>SRCTHLENRDFVTGTQGTTRVTLVLELGGCVTITAEGKPSMDVWLDAIYQENPAKTREYCLHAKLSDTKVAARCPTMGPATLAEEHQGGTVCKRDQSDRGWGNHCGLFGKGSIVACVKAACEAKKKATGHVYDANKIVYTVKVEPHTGDYVAANETHSGRKTASFTVSSEKTILTMGEYGDVSLLCRVASGVDLAQTVILELDKTVEHLPTAWQVHRDWFNDLALPWKHEGAQNWNNAERLVEFGAPHAVKMDVYNLGDQTGVLLKALAGVPVAHIEGTKYHLKSGHVTCEVGLEKLKMKGLTYTMCDKTKFTWKRAPTDSGHDTVVMEVTFSGTKPCRIPVRAVAHGSPDVNVAMLITPNPTIENNGGGFIEMQLPPGDNIIYVGELSHQWFQKGSSIGRVFQKTKKGIERLTVIGEHAWDFGSAGGFLSSIGKAVHTVLGGAFNSIFGGVGFLPKLLLGVALAWLGLNMRNPTMSMSFLLAGGLVLAMTLGVGA[3x];>[3x]TVRKERDGSTVIRAEGKDAATQVRVENGTCVILATDMGSWCDDSLSYECVTIDQGEEPVDVDCFCRNVDGVYLEYGRCGKQEGSRTRRSVLIPSHAQGELTGRGHKWLEGDSLRTHLTRVEGWVWKNKLLALAMVTVVWLTLESVVTRVAVLVVLLCLAPVYA

The envelope of immature TBEV particle contains 180 copies of each M protein precursor (prM) and E forming heterodimers. The prM protein stabilizes E, preventing premature virus activation and its fusion at low pH with the membranes of the trans-Golgi network (TGN). Flavivirus maturation occurs at mildly acidic pH, when host protease furin cleaves the prM protein to a pr peptide that will later dissociate from the particle and the M protein that remains in the particle, resulting in infectious viruses. Our atomic models of the major viral components, the E and prM proteins, indicate that the pr domains of prM have a critical role in holding the heterohexameric prM3E3 spikes in a metastable conformation.

(B) Atomic model of a Kuutsalo-14 prM3E3 spike refined against a 3.9-Å-resolution map. We observed a 1.0-Å root-mean-square deviation (RMSD) between Kuutsalo-14 and Neudoerfl atomic models for the Cα of prM and E ectodomains. The E ectodomains extend outward from the particle surface joining at the top like a tripod, with the pr domains of prM positioned at the top. The E-DII harboring the fusion loops join at the top of the prM3E3 spike and are capped by pr peptides, each of which binds to its respective E through an interface with a cumulative buried area of ~4700 Å2. The negatively charged prM surfaces cover the positively charged E-DII tips, obscuring the fusion loops. The heterohexamer structure of the spike is stabilized by pr-pr interactions, as direct E-E contacts in the spike are limited to just one small interaction surface of ~160 Å2. The two opposing prME dimers interact via a symmetrical pr-pr interface with ~460 Å2 buried surface area, involving hydrophobic residues Ala19, Ala20, Val31, Leu33, Val59, Val61, and Phe64 of both prM proteins. The third prME dimer joins from a side via a ~160-Å2 interface between its E protein and E from another dimer and a ~320-Å2 interface between its pr and E of another dimer. The residues forming the furin cleavage site are held in place by a polar interaction between Arg88 of pr and Glu243 of E, and is zipped downstream by the hydrophobic residues Val90, Leu91, and Ile92 of prM fitted into a hydrophobic pocket on E.> PLHS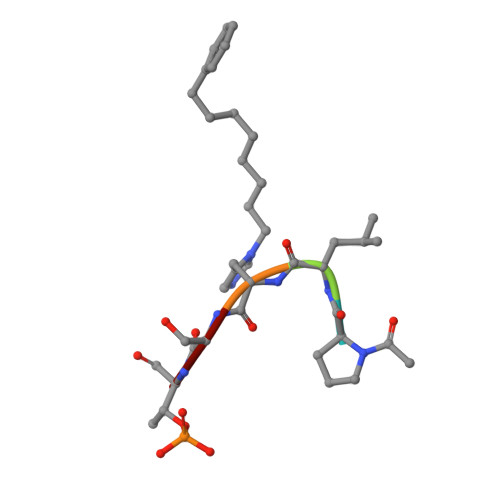T> SRHSCIF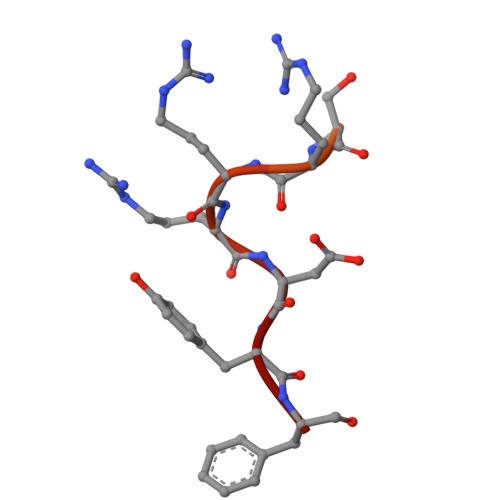PGQYNPSFISDESRRRDYF Prokaryotic type III CRISPR–Cas systems provide immunity against viruses and plasmids using CRISPR-associated Rossman fold (CARF) protein effectors. We studied WP_013033759 (hereafter named Cam1) from the halophilic Gram-negative chromatiaceae Nitrosococcus halophilus Nc4, which contains a CARF domain fused to a transmembrane domain that does not seem to be capable of degrading nucleic acids, as is the case for all the previously characterized CARF effectors. N. halophilus Cam1 (hereafter NhCam1) has a molecular mass of 22.3 kDa and contains 206 amino acids, with an N-terminal transmembrane helix (TMH) predicted to be 24 amino acids in length by deepTMHMM26 followed by an equally short linker (L1) and a C-terminal intracellular CARF domain. Here we investigated the structure and function of Cam1, a CARF effector that lacks a nuclease domain, but contains a TMH domain that promotes the formation of a tetrameric pore that is required to provide immunity through membrane depolarization and growth arrest of the infected cell (Supplementary Discussion).

We next grew crystals and solved the structure NhCam1-CARF (residues 42–206) in the absence and presence of bound cA4. The 2.2 Å-resolution X-ray structure without the ligand showed that NhCam1-CARF adopts a domain-swapped dimeric topology, in which the β7 strand of one monomer completes the folding topology of a second monomer by pairing with its β6 strand. Loop L2 connects β6 and β7 in one monomer, but this loop is disordered in the other monomer; loop L1 is disordered in both monomers of the CARF dimer. We identified 56 different Cam1 homologues, which we used to perform a MUSCLE protein sequence alignment, finding that D17, but not S24, is highly conserved. Notably, the apo NhCam1-CARF dimer crystal structure aligned to the CARF domain of the model with a root mean-squared deviation of 0.44 Å.

>[4x]SREDLRAWLTRNRFPRVGGVSESTVQWEGVVFTVSNESVPRWVMAQIQPAYMGLVATQASLAAAEAVAAVARRRGIEVHGPLQVADPNDPAASRSQVALLLSELRRAGCREIAVDLTGGKLPMSLGAFMAAEEAGVASLYVATDFDKHLKVPDMRTATLRQISQPE> TMSEIDRIAQNIIKSHLETCQYTMEELHQLAWQTHTYEEIKAYQSKSREALWQQCAIQITHAIQYVVEFAKRITGFMELCQNDQILLLKSGCLEVVLVRMCRAFNPLNNTVLFEGKYGGMQMFKALGSDDLVNEAFDFAKNLCSLQLTEEEIALFSSAVLISPDRAWLLEPRKVQKLQEKIYFALQHVIQKNHLDDETLAKLIAKIPTITAVCNLHGEKLQVFKQSHPDIVNTLFPPLYKELFN;> HKILHRL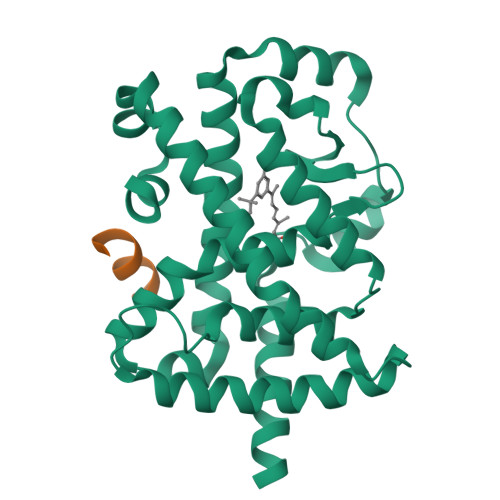LQE>[8x]MGRIKNKQFAVIGLGRFGGSICKELHRMGHEVLAVDINEEKVNAYASYATHAVIANATEENELLSLGIRNFEYVIVA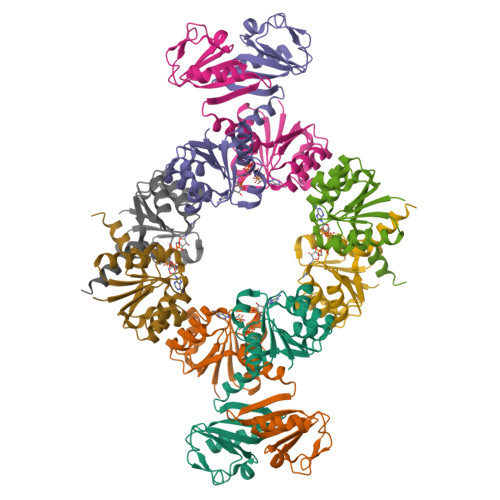IGANIQASTLTTLLLKELDIPNIWVKAQNYYHHKVLEKIGADRIIHPQKDMGVKIAQSLSDENVLNYIDLSDEYSIVELLATRKLDSKSIIDLNVRAKYGCTILAIKHHGDICLSPAPEDIIREQDCLVIMGHKKDIKRFENEGM> LPVLAPVTKDPATSLYTIPFHDGASLVLDVAGPLVWSTCDGGQPPAEIPCSSPTCLLANAYPAPGCPAPSCGSDKHDKPCTAYPYNPVSGACAAGSLSHTRFVANTTDGSKPVSKVNVGVLAACAPSKLLASLPRGSTGVAGLANSGLALPAQVASAQKVANRFLLCLPTGGPGVAIFGGGPVPWPQFTQSMPYTPLVTKGGSPAHYISARSIVVGDTRVPVPEGALATGGVMLSTRLPYVLLRPDVYRPLMDAFTKALAAQHANGAPVARAVEAVAPFGVCYDTKTLGNNLGGYAVPNVQLGLDGGSDWTMTGKNSMVDVKQGTACVAFVEMKGVAAGDGRAPAVI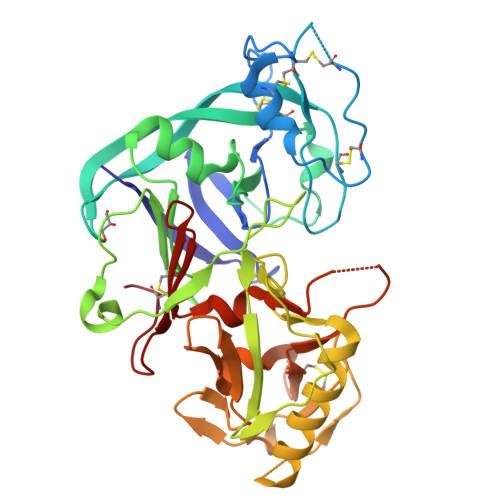LGGAQMEDFVLDFDMEKKRLGFSRLPHFTGCGGL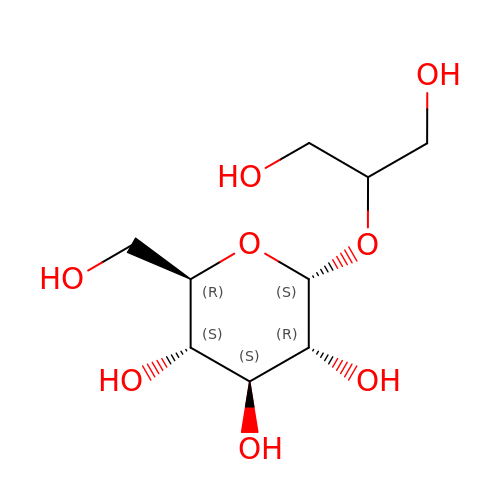1,3-dihydroxypropan-2-yl alpha-D-glucopyranoside | C9 H18 O8 | AQTKXCPRNZDOJU-ZEBDFXRSSA-N> MEKTRANSHLRSQPIDWTIEEVIQYIESNDNSLAVHGDLFRKHEIDGKALLRLNSERMMKYMGLKLGPALKICNLVNKVNGRDHHH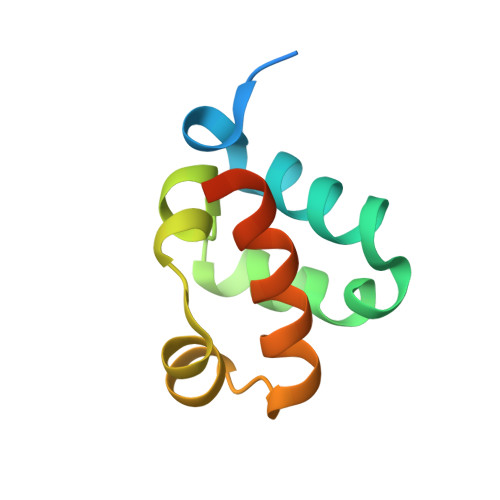HHH>[2x]GPGYQDPNNRYSFIGGRTGQWQVVKIRNVLGPGLQLVEKVNILNGAVAEIPLDSAWRLQGFASNIRYAIRTELEALQAVEPMLNRAEAI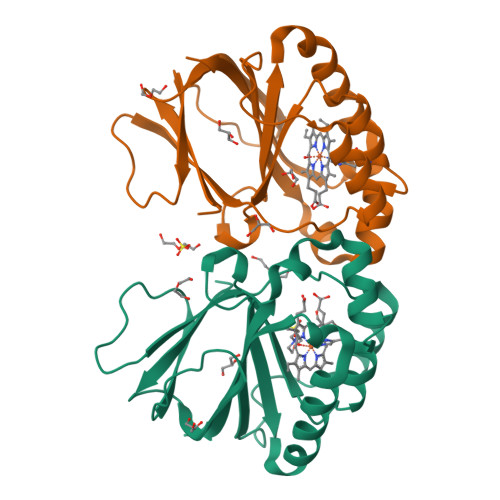LAVLIPIKKSAQWWEMAQDERRDIFERESHHTAVGLEYLPGVARRLLHCRDLGEEFDFLTWFEFAPEHSSAFNELLLRMRASKEWEYVEREVEVWLKRL> MEEQPQMQDADEPADSGGEGRAGGPPQVAGAQAACSEDRMTLLLRLRAQTKQQLLEYKSMVDASEEKTPEQIMQEKQIEAKIEDLENEIEEVKVAFEIKKLALDRMRLSTALKKNLEKISRQSSVLMDNMKHLLELNKLIMKSQQESWDLEEKLLDIRKKRLQLKQASESKLLEIQTEKNKQKIDLDSMENSERIKIIRQNLQMEIKITTVIQHVFQNLILGSKVNWAEDPALKEIVLQLEKNVDMM;> MSPQKRVKNVQAQNRTSQGSSSFQTTLSAWKVKQDPSNSKNISKHGQNNPVGDYEHADDQAEEDALQMAVGYFEKGPIKASQNKDKTLEKHLKTVENVAWKNGLASEEIDILLNIALSGKFGNAVNTRILKCMIPATVISEDSVVKAVSWLCVGKCSGSTKVLFYRWLVAMFDFIDRKEQINLLYGFFFASLQDDALCPYVCHLLYLLTKKENVKPFRVRKLLDLQAKMGMQPHLQALLSLYKFFAPALISVSLPVRKKIYFKNSENLWKTALLAVKQRNRGPSPEPLKLMLGPANVRPLKRKWNSLSVIPVLNSSSYTKECGKKEMSLSDCLNRSGSFPLEQLQSFPQLLQNIHCLELPSQMGSVLNNSLLLHYINCVRDEPVLLRFYYWLSQTLQEECIWYKVNNYEHGKEFTNFLDTIIRAECFLQEGFYSCEAFLYKSLPLWDGLCCRSQFLQLVSWIPFSSFSEVKPLLFDHLAQLFFTSTIYFKCSVLQSLKELLQNWLLWLSMDIHMKPVTNSPLETTLGGSMNSVSKLIHYVGWLSTTAMRLESNNTFLLHFILDFYEKVCDIYINYNLPLVVLFPPGIFYSALLSLDTSILNQLCFIMHRYRKNLTAAKKNELVQKTKSEFNFSSKTYQEFNHYLTSMVGCLWTSKPFGKGIYIDPEILEKTGVAEYKNSLNVVHHPSFLSYAVSFLLQESPEERTVNVSSIRGKKWSWYLDYLFSQGLQGLKLFIRSSVHHSSIPRAEGINCNNQY;> MNQEDLDPDSTTDVGDVTNTEEELIRECEEMWKDMEECQNKLSLIGTETLTDSNAQLSLLIMQVKCLTAELSQWQKKTPETIPLTEDVLITLGKEEFQKLRQDLEMVLSTKESKNEKLKEDLEREQRWLDEQQQIMESLNVLHSELKNKVETFSESRIFNELKTKMLNIKEYKEKLLSTLGEFLEDHFPLPDRSVKKKKKNIQESSVNLITLHEMLEILINRLFDVPHDPYVKISDSFWPPYVELLLRNGIALRHPEDPTRIRLEAFHQ;> MDSYSAPESTPSASSRPEDYFIGATPLQKRLESVRKQSSFILTPPRRKIPQCSQLQEDVDPQKVAFLLHKQWTLYSLTPLYKFSYSNLKEYSRLLNAFIVAEKQKGLAVEVGEDFNIKVIFSTLLGMKGTQRDPEAFLVQIVSKSQLPSENREGKVLWTGWFCCVFGDSLLETVSEDFTCLPLFLANGAESNTAIIGTWFQKTFDCYFSPLAINAFNLSWMAAMWTACKMDHYVATTEFLWSVPCSPQSLDISFAIHPEDAKALWDSVHKTPGEVTQEEVDLFMDCLYSHFHRHFKIHLSATRLVRVSTSVASAHTDGKIKILCHKYLIGVLAYLTELAIFQIE;> MSVLRPLDKLPGLNTATILLVGTEDALLQQLADSMLKEDCASELKVHLAKSLPLPSSVNRPRIDLIVFVVNLHSKYSLQNTEESLRHVDASFFLGKVCFLATGAGRESHCSIHRHTVVKLAHTYQSPLLYCDLEVEGFRATMAQRLVRVLQICAGHVPGVSALNLLSLLRSSEGPSLEDL;> MDETVAEFIKRTILKIPMNELTTILKAWDFLSENQLQTVNFRQRKESVVQHLIHLCEEKRASISDAALLDIIYMQFHQHQKVWEVFQMSKGPGEDVDLFDMKQFKNSFKKILQRALKNVTVSFRETEENAVWIRIAWGTQYTKPNQYKPTYVVYYSQTPYAFTSSSMLRRNTPLLGQALTIASKHHQIVKMDLRSRYLDSLKAIVFKQYNQTFETHNSTTPLQERSLGLDINMDSRIIHENIVEKERVQRITQETFGDYPQPQLEFAQYKLETKFKSGLNGSILAEREEPLRCLIKFSSPHLLEALKSLAPAGIADAPLSPLLTCIPNKRMNYFKIRDK;> MEQANPLRPDGESKGGVLAHLERLETQVSRSRKQSEELQSVQAQEGALGTKIHKLRRLRDELRAVVRHRRASVKACIANVEPNQTVEINEQEALEEKLENVKAILQAYHFTGLSGKLTSRGVCVCISTAFEGNLLDSYFVDLVIQKPLRIHHHSVPVFIPLEEIAAKYLQTNIQHFLFSLCEYLNAYSGRKYQADRLQSDFAALLTGPL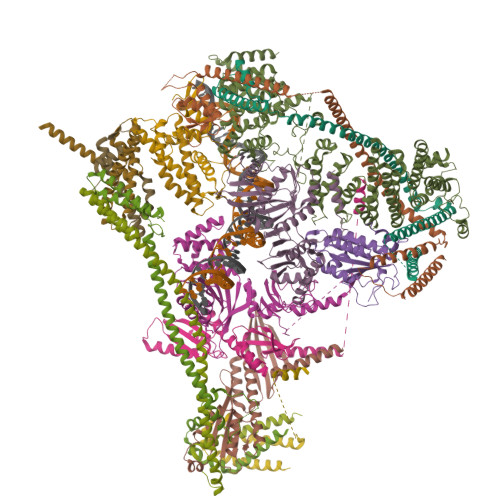QRNPLCNLLSFTYKLDPGGQSFPFCARLLYKDLTATLPTDVTVTCQGVEVLSTSWEEQRASHETLFCTKPLHQVFASFTRKGEKLDMSLVS;> MDAELAEVRALQAEIAALRRACEDPPAPWEEKSRVQKSFQAIHQFNLEGWKSSKDLKNQLGHLESELSFLSTLTGINIRNHSKQTEDLTSTEMTEKSIRKVLQRHRLSGNCHMVTFQLEFQILEIQNKERLSSAVTDLNIIMEPTECSELSEFVSRAEERKDLFMFFRSLHFFVEWFEYRKRTFKHLKEKYPDAVYLSEGPSSCSMGIRSASRPGFELVIVWRIQIDEDGKVFPKLDLLTKVPQRALELDKNRAIETAPLSFRTLVGLLGIEAALESLIKSLCAEENN;> MSGKANASKKNAQQLKRNPKRKKDNEEVVLSENKVRNTVKKNKNHLKDLSSEGQTKHTNLKHGKTAASKRKTWQPLSKSTRDHLQTMMESVIMTILSNSIKEKEEIQYHLNFLKKRLLQQCETLKVPPKKMEDLTNVSSLLNMERARDKANEEGLALLQEEIDKMVETTELMTGNIQSLKNKIQILASEVEEEEERVKQMHQINSSGVLSLPELSQKTLKAPTLQKEILALIPNQNALLKDLDILHNSSQMKSMSTFIEEAYKKLDAS;> MPVKRSLKLDGLLEENSFDPSKITRKKSVITYSPTTGTCQMSLFASPTSSEEQKHRNGLSNEKRKKLNHPSLTESKESTTKDNDEFMMLLSKVEKLSEEIMEIMQNLSSIQALEGSRELENLIGISCASHFLKREMQKTKELMTKVNKQKLFEKSTGLPHKASRHLDSYEFLKAILN;> MEEEAETEEQQRFSYQQRLKAAVHYTVGCLCEEVALDKEMQFSKQTIAAISELTFRQCENFAKDLEMFARHAKRTTINTEDVKLLARRSNSLLKYITDKSEEIAQINLERKAQKKKKSEDGSKNSRQPAEAGVVESEN;> MADHNPDSDSTPRTLLRRVLDTADPRTPRRPRSARAGARRALLETASPRKLSGQTRTIARGRSHGARSVGRSAHIQASGHLEEQTPRTLLKNILLTAPESSILMPESVVKPVPAPQAVQPSRQESSCGSLELQLPELEPPTTLAPGLLAPGRRKQRLRLSVFQQGVDQGLSLSQEPQGNADASSLTRSLNLTFATPLQPQSVQRPGLARRPPARRAVDVGAFLRDLRDTSLAPPNIVLEDTQPFSQPMVGSPNVYHSLPCTPHTGAEDAEQAAGRKTQSSGPGLQKNSPGKPAQFLAGEAEEVNAFALGFLSTSSGVSGEDEVEPLHDGVEEAEKKMEEEGVSVSEMEATGAQGPSRVEEAEGHTEVTEAEGSQGTAEADGPGASSGDEDASGRAASPESASSTPESLQARRHHQFLEPAPAPGAAVLSSEPAEPLLVRHPPRPRTTGPRPRQDPHKAGLSHYVKLFSFYAKMPMERKALEMVEKCLDKYFQHLCDDLEVFAAHAGRKTVKPEDLELLMRRQGLVTDQVSLHVLVERHLPLEYRQLLIPCAYSGNSVFPAQ;> MAPRGRRRPRPHRSEGARRSKNTLERTHSMKDKAGQKCKPIDVFDFPDNSDVSSIGRLGENEKDEETYETFDPPLHSTAIYADEEEFSKHCGLSLSSTPPGKEAKRSSDTSGNEASEIESVKISAKKPGRKLRPISDDSESIEESDTRRKVKSAEKISTQRHEVIRTTASSELSEKPAESVTSKKTGPLSAQPSVEKENLAIESQSKTQKKGKISHDKRKKSRSKAIGSDTSDIVHIWCPEGMKTSDIKELNIVLPEFEKTHLEHQQRIESKVCKAAIATFYVNVKEQFIKMLKESQMLTNLKRKNAKMISDIEKKRQRMIEVQDELLRLEPQLKQLQTKYDELKERKSSLRNAAYFLSNLKQLYQDYSDVQAQEPNVKETYDSSSLPALLFKARTLLGAESHLRNINHQLEKLLDQG;> MALSTIVSQRKQIKRKAPRGFLKRVFKRKKPQLRLEKSGDLLVHLNCLLFVHRLAEESRTNACASKCRVINKEHVLAAAKVILKKSRG;> MEGAGAGSGFRKELVSRLLHLHFKDDKTKVSGDALQLMVELLKVFVVEAAVRGVRQAQAEDALRVDVDQLEKVLPQLLLDF>[6x]EKDPLWLYKVLLTKGIEVWFDIKLEKYGIKRNNRVDYIAKSSLQQIVFEIIGKTPKNIAVPTYIGAYEPSKPEKWEEEGIKYINLFKPTPLMKVKPVKEMPEIVKNLLLNLFDYDAKSMGLFINWLAFIYQYKERTGVAWIFMGKQGTGKGLLVDLLKKIFEEHMSSNITDANLDSQFNPYLYNKLIVHLNEVSADNRKSRMLVKNRLKTWITDETLYINRKNMKEVEIKNFCNFIINSNETIPVDIEDSDRRFNVIECNNVLKEQEWWTTESYQEILNNAEGFAKYLAGIKVDRSKVNEVVMSEKKKAIVETTESVLKQIAKALTDRDIEWFLDNGLEGVVEKNIVNDFQWEELQEAITTGVIPNKYLMIIVEQILGDSKTITWIKRNIITPYQVGETTVVKMAGKPIRAIVVG

NrS-1 polymerase is a multidomain enzyme and is one key component of the phage replisome. The N-terminal Prim/Pol and HBD domains are responsible for DNA polymerization and de novo primer synthesis activities of NrS-1 polymerase. Here, we report two crystal structures, showing that NrS-1 CTR adopts one unique hexameric ring-shaped conformation. Although the central helicase domain of NrS-1 CTR shares structural similarity with the superfamily III helicases, the folds of the Head and Tail domains are completely novel.

Totally, two NrS-1 CTR structures were determined, one in A-form and another in B-form. The A-form crystals were grown in P212121 space group; per asymmetric unit contains six copies of NrS-1 CTR monomer, which were assembled into a ring-shaped architecture. NrS-1 CTR assembles into ring-shaped hexamer in both structures. The helicase domain forms hexameric ring in both A- and B-form NrS-1 CTR structures. NrS-1 CTR forms hexamer in both A- and B-form structures, however, as confirmed by the size-exclusion chromatographic analysis, NrS-1 N618 exists as a monomer.> MKTVALILASLALLACTAESGVDF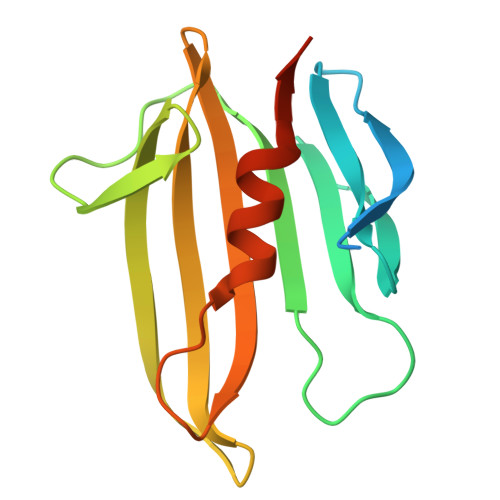DKTLTHPNGLVVERPVGFDARRSAEGFRFDEGGKLRNPRQLEVQRQDAPPPPDLASRRLGDGEARYKVEEDDGGSAGSEYRLWAAKPAGARWIVVSASEQSEDGEPTFALAWALLERARLQLEHHHHHH2'-azido-2'-deoxycytidine 5'-(dihydrogen phosphate) | C9 H13 N6 O7 P | 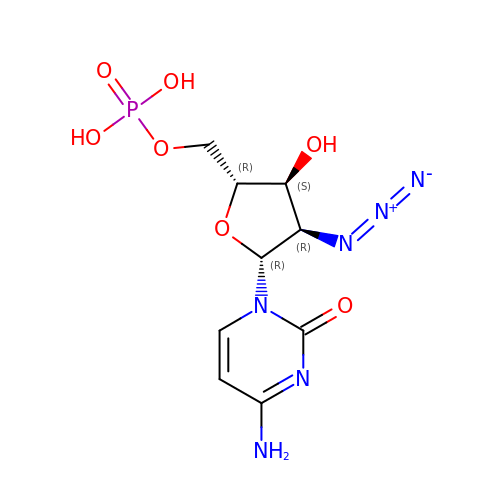GXKFYGVDGIPSIP-XVFCMESISA-N>MADKIKDAKIIFVVGGPGSGKGTQCEKVVAKYGYTH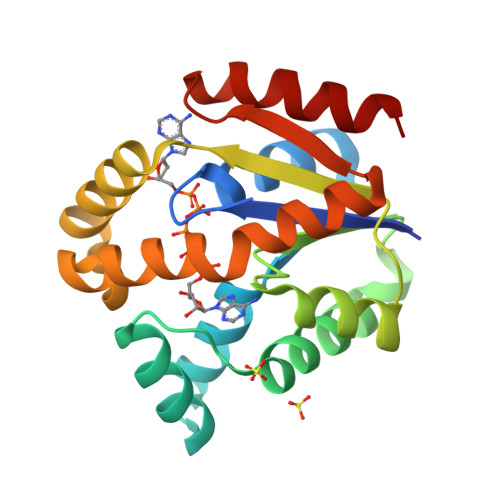LSSGDLLRAEVSSGSERGKQLQAIMQKGELVPLDTVLDMIKDAMIAKADVSKGYLIDGYPREVKQGEEFEKKIGKPCLLLYIDAKGETMVKRLMKRGETSGRADDNEETIKKRLDLYYKATEPVIAFYEGRGIVRKVDSELPVDEVFKQVSTAIDAL[2x]>[2x]MGKYFGTDGVRGVANQELTPELAFKLGRYGGYVLAHNKGEKHPRVLVGRDTRVSGEMLESALIAGLISIGAEVMRLGIISTPGVAYLTRDMGAELGVMISASHNPVADNGIKFFGSDGFKLSDEQENEIEALLDQENPELPRPVGNDIVHYSDYFEGAQKYLSYLKSTVDVNFEGLKIALDGANGSTSSLAPFLFGDLEADTETIGCSPDGYNINEKCGSTHPEKLAEKVVETESDFGLAFDGDGDRIIAVDENGQIVDGDQIMFIIGQEMHKNQELNNDMIVSTVMSNLGFYKALEQEGIKSNKTKVGDRYVVEEMRRGNYNLGGEQSGHIVMMDYNTTGDGLLTGIQLASVIKMTGKSLSELAGQMKKYPQSLINVRVTDKYRVEENVDVKEVMTKVEVEMNGEGRILVRPSGTEPLVRVMVEAATDEDAERFAQQIADVVQDKMGLDKLVPR

In the human pathogen Staphylococcus aureus, c-di-AMP is produced by the di-adenylate cyclase enzyme DacA, which is thought to form a complex and be regulated by YbbR and GlmM, two other conserved proteins. GlmM codes for the essential phosphoglucosamine mutase enzyme, required for the conversion of glucosamine-6-phosphate to the early peptidoglycan synthesis precursor glucosamine-1-phosphate. We determined the atomic structures of the S. aureus DacA and GlmM enzymes and show that GlmM readily binds to DacA in vitro and blocks its activity by masking its active site. Specifically, our data suggest that GlmM blocks access to the active site of DacA and in this manner prevents the formation of catalytically active head-to-head DacA oligomers.

In order to gain structural information on the S. aureus DacACD/GlmM complex, we first set out to determine the structure of the S. aureus GlmM protein in isolation. While the protein was crystallized in the presence of metal ion and substrate, no corresponding extra electron density was observed. The S. aureus GlmM protein and the B. anthracis protein, which share 67% identity on a protein level, displayed a similar fold and dimeric arrangement and the structures overlapped with an RMSD of 0.996 Å. One GlmM monomer consisted of four α-β domains with the fourth most C-terminal domain linked by a flexible loop. The reconstructed model for the GlmM sample showed an elongated particle, consistent with the dimeric arrangement found in the crystal structure and with previously published findings. A sequential fitting of the GlmM dimer structure followed by the fitting of the DacA dimer structure into the SAXS envelope of the complex with Chimera yielded the best fit for a model with a correlation score of 0.9196 in which a DacA dimer is positioned on top of a GlmM dimer. In this model, the active sites of DacA protomers are occluded through binding to the GlmM protein, while the GlmM active sites are still accessible. In our model, the DacACD active sites in both protomers are capped by the α5 helix of GlmM and neighbouring residues. Interestingly, positioned next to the α5 helix in GlmM is residue F155, which in a previous study was shown to modulate the GlmM-CdaA interaction in L. lactis. Upon binding, GlmM completely abolished the activity of the DacA cyclase enzyme, while GlmM activity was not significantly affected upon complex formation.> DKKPPPYKHIKVNRPIGRVQIFTADLSEIPRCNCKATDENPCGIDSECINRMLLYECHPTVCPAGGRCQNQCFSKRQYPEVEIFRTLQRGWGLRTKTDIKKGEFVNEYVGELIDEEECRARIRYAQEHDITNFYMLTLDKDR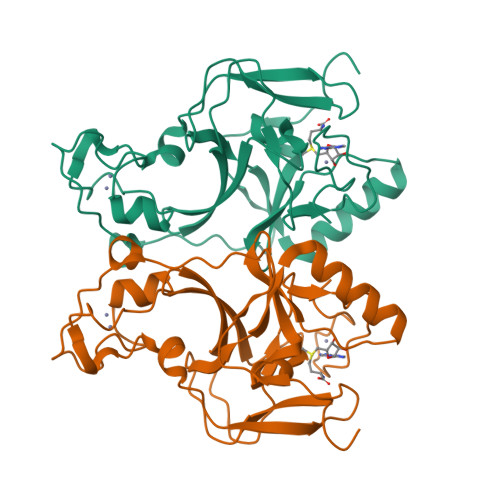IIDAGPKGNYARFMNHCCQPNCETQKWSVNGDTRVGLFALSDIKAGTELTFNYNLECLGNGKTVCKCGAPNCSGFLGV4-(6-CHLORO-2,4-DIOXO-1,2,3,4-TETRAHYDROPYRIMIDIN-5-YL) BUTYL PHOSPHATE 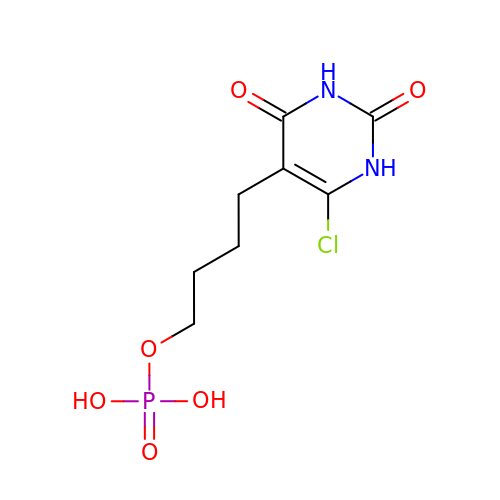| C8 H12 Cl N2 O6 P | DAUATIBSDSXXHA-UHFFFAOYSA-N> HMMATGDERFYAEHLMPTLQGLLDPESAHRLAVRFTSLGLLPRARFQDSDMLEVRVLGHKFRNPVGIAAGFDKHGEAVDGLYKMGFGFVEIGSVTPKPQEGNPRPRVFRLPEDQAVINRYGFNSHGLSVVEHRLRARQQKQAKLTEDGLPLGVNLGKNKTSVDAAEDYAEGVRVLGPLADYLVVNVSSPNTAGLRSLQGKAELRRLLTKVLQERDGLRRVHRPAVLVKIAPDLTSQD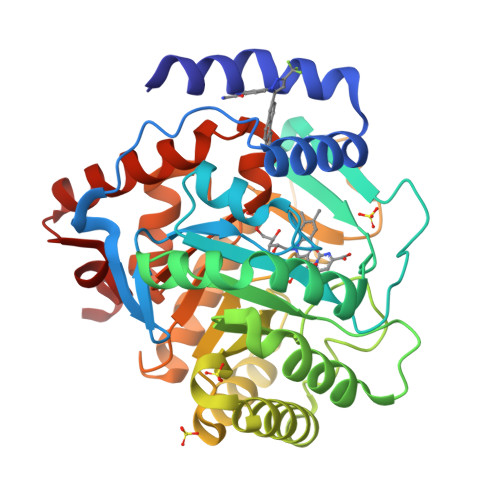KEDIASVVKELGIDGLIVTNTTVSRPAGLQGALRSETGGLSGKPLRDLSTQTIREMYALTQGRVPIIGVGGVSSGQDALEKIRAGASLVQLYTALTFWGPPVVGKVKRELEALLKEQGFGGVTDAIGADHRR5-chloranyl-6-(4-fluorophenyl)-8-oxidanyl-3~{H}-quinazolin-4-one | 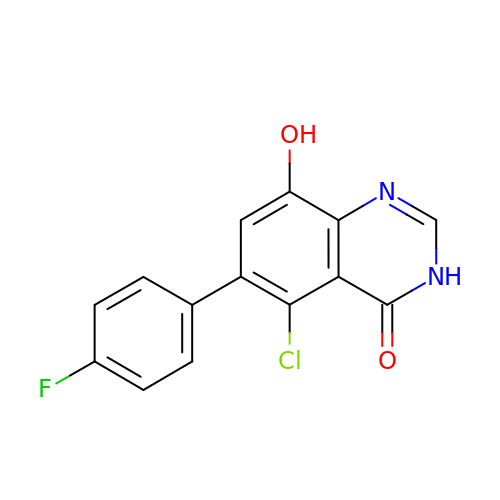C14 H8 Cl F N2 O2 | ZRBUMFCLSOEMBA-UHFFFAOYSA-N> HHHHHHMAEQVKLSVELIACSSFTPPADVEWSTDVEGAEALVEFAGRACYETFDKPNPRTASNAAYLRHIMEVGHTALLEHANATMYIRGISRSATHELVRHRHFSFSQLSQRFVHSGESEVVVPTLIDEDPQLRELFMHAMDESRFAFNELLNALEEKLGDEPNALLRKKQARQAARAV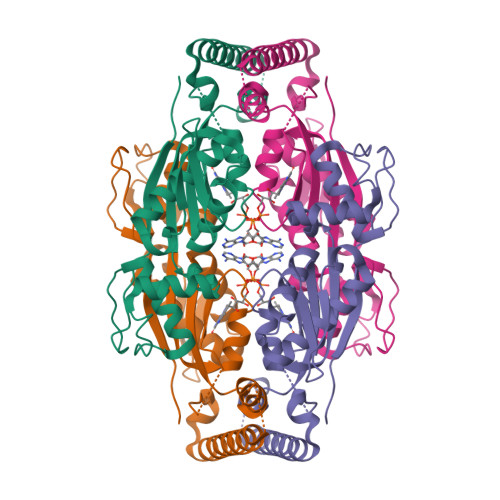LPNATESRIVVSGNFRTWRHFIGMRASEHADVEIREVAVECLRKLQVAAPTVFGDFEIETLADGSQMATSPYVMDF The semaphorins are the largest family of evolutionarily conserved axon guidance cues. The semaphorins signal through their main receptors, plexins, which are single-spanning transmembrane proteins expressed in a variety of cell types, including neurons, cancer cells or endothelial cells. We determined crystal structures of Drosophila Sema1a1–2, Sema1b1–2, Sema2a1–3 and Sema2b1–3 to a 3.6-, 2.8-, 2.1- and 2.5 -Å resolution, respectively. All structures contain the sema domain composed of a seven-bladed β-propeller fold, which is followed by a PSI domain.

The secreted semaphorins Sema2a and Sema2b also contain an Ig-like domain positioned C-terminally to their PSI domains. Sema2a and Sema2b are very similar and share over 67% sequence identity. A superposition of Sema2a1–3 and Sema2b1–3 crystal structures unveiled that Sema2a and Sema2b are also highly similar in structure with an rmsd of 1.1 Å over 608 Cα atoms (for Sema2a chain A and Sema2b chain A). Most notable variations are observed in the distribution of charged patches located on their surfaces. On the other hand, when we mutated the equivalent cysteine residue to serine in Sema2afull and Sema2bfull, both proteins partially maintained the homodimeric architecture and a mixture of a monomer and a non-covalent dimer was observed. However, this distinctive glycan is also well-ordered in the Sema1b and Sema2b structures. Within classes, Sema2b binds PlexB ~8 times more strongly than Sema2a. Given the essentially identical architecture of Sema2a and Sema2b, we conclude that their different binding properties either in strength or lifetime of binding to PlexB or interaction with additional co-receptor, determine their distinct functions.

>ETGYENTWNLYYEPPCCTGSSAAHHLRHHKEHVQDFSCGPLHYKTFYMDERNNALYVGAMDRIFRLNLRNISQSICERDVLILEPTGSDILNCVSKGKREKVECRNHIRVIQPMNFNGQKLYVCGTNAHNPKDYVINANLTHLPRSQYVPGIGLGIGKCPYDPADNSTAVYVENGNPFGLPALYAGTNAEFTKADSVIFRSDLYNLTNGRKEANFKRTVKYDSKLLDKPNFVGSFEIGEFVYFFFREHAVEYINCGKAVYSRVARVCKNDRGGKYMISQNWATYLKARMNCSISSEFPFYFNEIQSVYKMPTDDTKFYATFTTNTNGLIGSAVCSYDIRDINAAFDGKFKEQATSNSAWLPVLNSKVPEPRPGTCHNDTATLPDSVLNFIRKHPLMDKAVDHEFGNPVFFKRDVILTKLVVDKIRIDKLNQEFLVYFVATTSGHIYKIVQFMHYGQRHSNLVDIFEASPHSEPIREMTLSHKTGSLYVATDHQVKQIDIAMCARRYDSCFRCVSDPYCGWDKDVNACRPYQLGLLQDVANETSGICDTSVLRKKVTSSYGQTLHLSCFVKMPEVLRKKQTRWYHHSTEKGRYEVRYTPTKYIDTNEGGLVLLAVNEGDGGRYDSYLDGTLLCSYGVTVDAHRCSPPSQGTKHHHHHH[2x]>[2x]GAUUUGGGGAGUAGCCGAUUUCCGAAAGGAAAUGUACGUGUC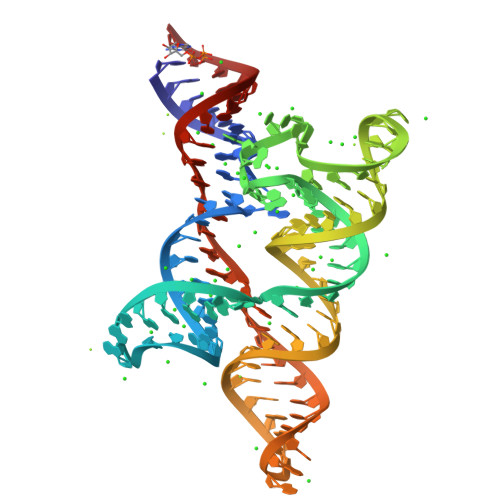AACAUUUUCGUUGAAAAACGUGGCACGUACGGACUGAAGAAAUUCAGUCAGGCGAGACCAUAUCC> MTPLRVFRKTTPLVNTIRLSLLPLAGLSFSAFAAQVNIAPGSLDKALNQYAAHSGFTLSVDASLTRGKQ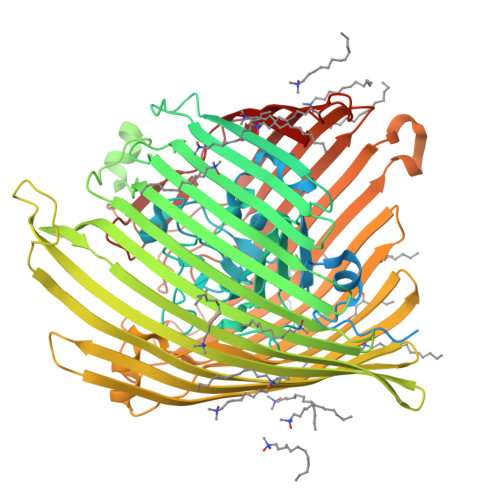SNGLHGDYDVESGLQQLLDGSGLQVKPLGNNSWTLEPAPAPKEDALTVVGDWLGDARENDVFEHAGARDVIRREDFAKTGATTMREVLNRIPGVSAPENNGTGSHDLAMNFGIRGLNPRLASRSTVLMDGIPVPFAPYGQPQLSLAPVSLGNMDAIDVVRGGGAVRYGPQSVGGVVNFVTRAIPQDFGIEAGVEGQLSPTSSQNNPKETHNLMVGGTADNGFGTALLYSGTRGSDWREHSATRIDDLMLKSKYAPDEVHTFNSLLQYYDGEADMPGGLSRADYDADRWQSTRPYDRFWGRRKLASLGYQFQPDSQHKFNIQGFYTQTLRSGYLEQGKRITLSPRNYWVRGIEPRYSQIFMIGPSAHEVGVGYRYLNESTHEMRYYTATSSGQLPSGSSPYDRDTRSGTEAHAWYLDDKIDIGNWTITPGMRFEHIESYQNNAITGTHEEVSYNAPLPALNVLYHLTDSWNLYANTEGSFGTVQYSQIGKAVQSGNVEPEKARTWELGTRYDDGALTAEMGLFLINFNNQYDSNQTNDTVTARGKTRHTGLETQARYDLGTLTPTLDNVSIYASYAYVNAEIREKGDTYGNLVPFSPKHKGTLGVDYKPGNWTFNLNSDFQSSQFADNANTVKESADGSTGRIPGFMLWGARVAYDFGPQMADLNLAFGVKNIFDQDYFIRSYDDNNKGIYAGQPRTLYMQGSLKF> PISPIETVPVKLKPGMDGPKVKQWPLTEEKIKALVEICTEMEKEGKISKIGPENPYNTPVFAIKKKDSTKWRKLVDFRELNKRTQDFWEVQLGIPHPAGLKKKKSVTVLDVGDAYFSVPLDEDFRKYTAFTIPSINNETPGIRYQYNVLPQGWKGSPAIFQSSMTKILEPFKKQNPDIVIYQYMDDLYVGSDLEIGQHRTKIEELRQHLLRWGLTTPDKKHQKEPPFLWMGYELHPDKWTVQPIVLPEKDSWTVNDIQKLVGKLNWASQIYPGIKVRQLCKLLRGTKALTEVIPLTEE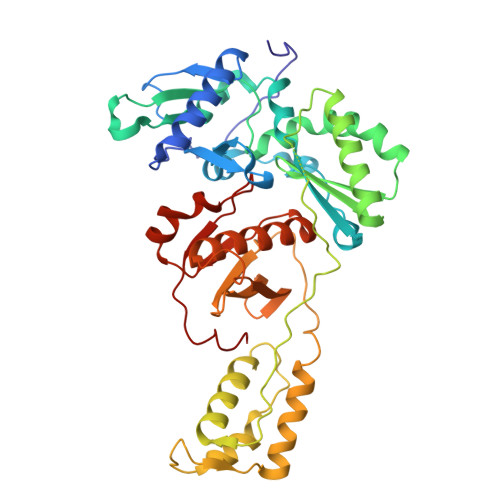AELELAENREILKEPVHGVYYDPSKDLIAEIQKQGQGQWTYQIYQEPFKNLKTGKYARMRGAHTNDVKQLTEAVQKITTESIVIWGKTPKFKLPIQKETWETWWTEYWQATWIPEWEFVNTPPLVKLWY>MRGSHHHHHHGSMREYTSKKELKEEIEKKYEKYDAEFETISESQKDEKVETVDRTPSENLSYQLGWVNLLLEWEAKEIAGYNVETPAPGYKWNNLGGLYQSFYKKYGIYSIKEQRAKLREAVNEVYKWISTLSDDELFQAGNRKWATT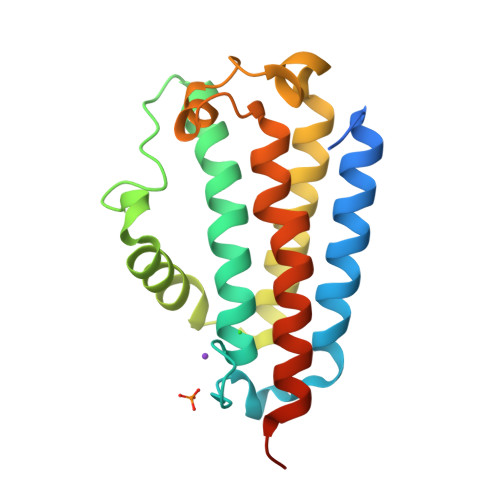KAMWPVYKWIHINTVAPFTNFRGKIRKWKRLVPEEQRIKRRKI[2x]Among the best characterized of the CYP152 family peroxygenases is the industrially relevant OleTJE (CYP152L1), first isolated from Jeotgalicoccus sp. ATCC 8456 in 2011 by Schirmer and co-workers. OleTJE acts primarily as a H2O2-dependent fatty acid decarboxylase to form terminal alkenes but also hydroxylates a proportion of these substrates to generate α- and β-hydroxylated fatty acids. Crystal structure data show that the active sites of OleTJE and P450 BSβ are very similar, with the carboxylate group of fatty acid substrates being coordinated by a conserved arginine residue (Arg245 in OleTJE, Arg242 in P450 BSβ, and Arg241 in P450 SPα). In this study, we explore further the structure and mechanism of OleTJE by mutating the key active site residues His85, Phe79, and Arg245 and by analyzing their effects on the catalytic properties of this biotechnologically important alkene-producing enzyme.

The H85Q mutant was characterized to establish whether His85 is crucial to OleTJE decarboxylase activity and also because its replacement by Glu85 in P450 BSβ results mainly in fatty acid hydroxylation. Crystals were obtained for both the H85Q and F79A mutant P450s in complex with arachidic acid substrate, as well as for the WT OleTJE in conditions containing formate. Structures for these mutant enzymes were determined to 1.44 Å (WT/formate), 1.80 Å (H85Q/arachidic acid) and 1.95 Å (F79A/arachidic acid). Arachidic acid substrate is bound similarly in both the H85Q and F79A mutants as was previously reported for the WT OleTJE. In contrast, for both OleTJE H85Q/F79A mutant structures, a sixth ligand water molecule is clearly visible. The H85Q mutant was found to generate a product profile very similar to that for the wild type OleTJE for all substrates tested. However, UV-visible binding studies demonstrate that substrate-induced H85Q HS heme accumulation is much lower than in the WT OleTJE in all cases. The LS heme iron signals for the H85Q mutant are quite distinct from those for WT OleTJE in both the substrate-free and arachidic acid-bound forms, indicating that the H85Q mutation alters the environment of the distal pocket around the heme iron, e.g. through altering the hydrogen bonding network to the distal water ligand in the LS substrate-free form. The similarity in product profiles between WT and H85Q OleTJE suggests that His85 is not crucial for proton transfer to transient heme iron-oxo species to facilitate C–C bond scission and alkene production or that alternative pathway(s) exist in the H85Q mutant. The data appear to rule out a key role for His85 in proton donation to reactive iron-oxo species in OleTJE, and suggest that the system is robust and that alternative protonation pathway(s) may exist.

> MATLKRDKGLDNTLKVLKQGYLYTTNQRNRLNTSVFQTKALGGKPFVVVTGKEGAEMFYNNDVVQREGMLPKRIVNTLFGKGAIQTVDGKKHVDRKALFMSLMTEGNLNYVRELTRTLWHANTQRMESMDEVNIYRESIVLLTKVGTRWAGVQAPPEDIERIATDMDIMIDSFRALGGAFKGYKASKEARRRVEDWLEEQIIETRKGNIHPPEGTALYEFAHWEDYLGNPMDSRTCAIDLMNTFRPLIAINRFVSFGLHAMNENPITREKIKSEPDYAYKFAQEVRRYYPFVPFLPGKAKVDIDFQGVTIPAGVGLALDVYGTTHDESLWDDPNEFRPERFETWDGSPFDLIPQGGGDYWTNHRCAGEWITVIIMEETMKYFAEKITYDVPEQDLEVDLNSIPGYVKSGFVIKNVREVVDRT;> HHHHHHMATLKRDKGLDNTLKVLKQGYLYTTNQRNRLNTSVFQTKALGGKPFVVVTGKEGAEMFYNNDVVQREGMLPKRIVNTLFGKGAIQTVDGKKHVDRKALFMSLMTEGNLNYVRELTRTLWHANTQRMESMDEVNIYRESIVLLTKVGTRWAGVQAPPEDIERIATDMDIMIDSFRALGGAFKGYKASKEARRRVEDWLEEQIIETRKGNIHPPEGTALYEFAHWEDYLGNPMDSRTCAIDLMNTFRPLIAINRFVSFGLHAMNENPITREKIKSEPDYAYKFAQEVRRYYPFVPFLPGKAKVDIDFQGVTIPAGVGLALDVYGTTHDESLWDDPNEFRPERFETWDGSPFDLIPQGGGDYWTNHRCAGEWITVIIMEETMKYFAEKITYDVPEQDLEVDLNSIPGYVKSGFVIKNVREVVDRT Tailoring steps catalyzed by SAM methyltransferase-like proteins have yielded particular insight into evolution of anthracyclines and generation of structural diversity. DnrK is a canonical S-adenosyl-L-methionine (SAM)-dependent methyltransferase that catalyzes 4-O-methylation in daunorubicin biosynthesis. Recent studies have uncovered that DnrK is bifunctional and catalyzes additional 10-decarboxylation as a moonlighting activity. Here we have taken advantage of the natural diversity of anthracycline methyltransferases and employed extensive chimeragenesis to probe factors that govern catalysis and substrate recognition.

The specificity of EamK and related 10-decarboxylase TamK lies between DnrK and RdmB, since anthracycline aglycones and monoglycosylated compounds are accepted as substrates. TamK has been shown to catalyze 10-decarboxylation of 4 and 5, but not 6 (29). The SAM binding site is highly conserved in the enzyme family with the exception of the 10-decarboxylases that contain two mutations G189A/K190P. The structure of the binary complex of wild-type TamK and SAM confirmed the interactions between the co-substrate and R4 in 10-decarboxylases. The overall fold of TamK remains very similar to that of the other members of the family with modest root-mean-square deviations to DnrK (3.7 Å) and to RdmB (3.8 Å). However, the distinct proline-alanine pair in R4 alters the conformation of the Cα main chain in the region and leads to a movement of 2.1 Å in comparison to DnrK. This change coincides with a 1.8 Å change in SAM positioning, which is the most likely reason behind the lack of methylation activity in TamK. Two-point mutations G189A/K190P in R4 are sufficient for misalignment of SAM and loss-of-methylation activity.

> MAHHHHHHHRSSGTDAGTAGTAGTAGAGAGGDRQHVDALVRMSNLVTPMALRVAATLRLVDHLRAGATSADALADATGADADALARLMRHLAAAGVLEEPEPGHYAPTGLGDLLADDHPSRQRSWLDLDQAVGRADLTFLGLREAVRTGRPQYEARYGKPFWTDLSEDDGLGASFDALMTTREDTAFAAPVAAYDWTRARHVLDVGGAPGGLLTAILRAAPEAHGTLLDLPGAAARTRERIAANGMDERIDVVGGDFFDELPVTADVVVLSFTLLNWSDPDALRILGRCRDALRPGGRIVLLERAEAPSGGTRTSDLYFSVLDMRMLVFLGGRVRTDREWADLAAAAGLDIVGKTGPLVSPNVPLDSCLWELAPR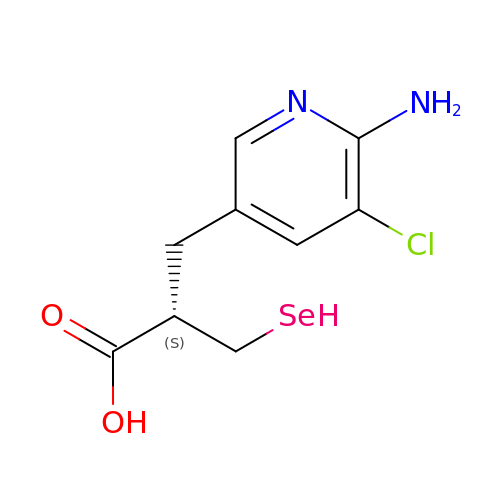(2~{S})-2-[(6-azanyl-5-chloranyl-pyridin-3-yl)methyl]-3-selanyl-propanoic acid | C9 H11 Cl N2 O2 Se | ZMJHVPIYUURBAQ-ZCFIWIBFSA-N>EDICFIAGIGDTNGYGWGIAKELSKRNVKIIFGIWPPVYNIFMKNYKNGKFDNDMIIDKDKKMNILDMLPFDASFDTANDIDEETKNNKRYNMLQNYTIEDV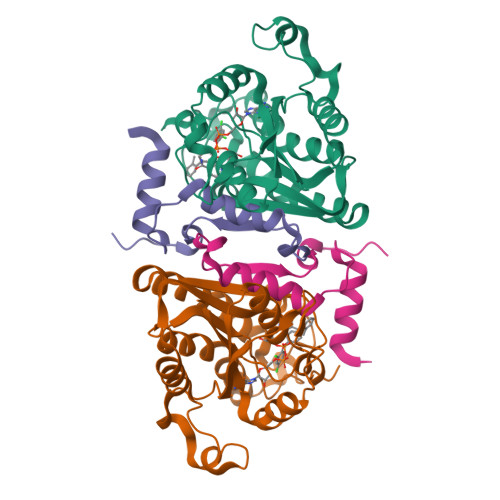ANLIHQKYGKINMLVHSLANAKEVQKDLLNTSRKGYLDALSKSSYSLISLCKYFVNIMKPQSSIISLTYHASQKVVPGYGGGMSSAKAALESDTRVLAYHLGRNYNIRINTISAGPLKSRAATAINKLNNTYENNTNQNKNRNSHDVHNIMNNSGEKEEKKNSASQN[2x];>YTFIDYAIEYSEKYAPLRQKLLSTDIGSVASFLLSRESRAITGQTIYVDNGLNIMFLPDD[2x]>[4x]MGSSHHHHHHSSDHRKIGRDQELYFFHELSPGSCFFLPKGAYIYNALIEFIRSEYRKRGFQEVVTPNIFNSRLWMTSGHWQHYSENMFSFEVEKELFALKPMNCPGHCLMFDHRPRSWRELPLRLADFGVLHRNELSGALTGLTRVRRFQQDDAHIFCAMEQIEDEIKGCLDFLRTVYSVFGFSFKLNLSTRPEKFLGDIEVWDQAEKQLENSLNEFGEKWELNSGDGAFYGPKIDIQIKDA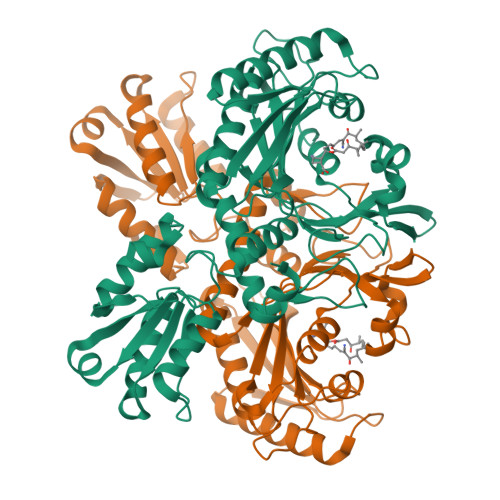IGRYHQCATIQLDFQLPIRFNLTYVSHDGDDKKRPVIVHRAILGSVERMIAILTENYGGKWPFWLSPRQVMVVPVGPTCDEYAQKVRQQFHDAKFMADIDLDPGCTLNKKIRNAQLAQYNFILVVGEKEKISGTVNIRTRDNKVHGERTISETIERLQQLKEFRSKQAEEEF>ASPELSALEEAFRRFAVHGDARATGREMHGKNWSKLCKDCQVIDGRNVTVTDVDIVFSKIKGKSCRTITFEQFQEALEELAKKRFKDKSSE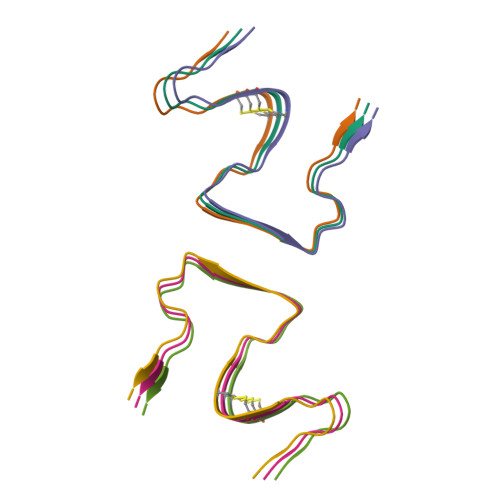EAVREVHRLIEGKAPIISGVTKAISSPTVSRLTDTTKFTG[6x]> MYRYEKKGPKRGVALYSYSAEFGLTKTLEDCFEDLHDMGAHGIEILANTHIENYPYPTDEWVEKWWRLCDKYEIVPVEYGNWIDSHVLGDRDLTTEESVEMLKRDIRLAHRLGFTVMRTKMPVINDLLEPVENWKEIIKGALPLAEELGIKMCPEIHTPSNLKGKLVNDFVEFIKETGTKNFGLNIDFSVFRTSFAEGEWVDPNYTPNKPEDIIPLLPYVYCCHAKFIHMSDDFKETTIPYEEVVKTMEDN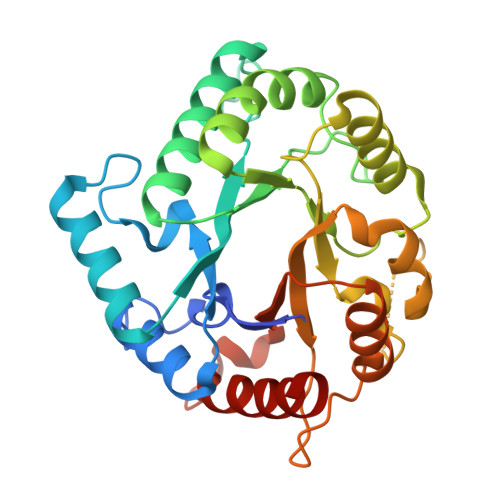GYEGYLLSEYEGADKYDEGYEVGQTLRKHHILLKNLLGD>GEDPQTFEGAGVVFEVQVEKNLVDIDHRLYRLPNSTVRNGMPSLFQVKPGSVVSYSGTVSQPWSTITDIYIH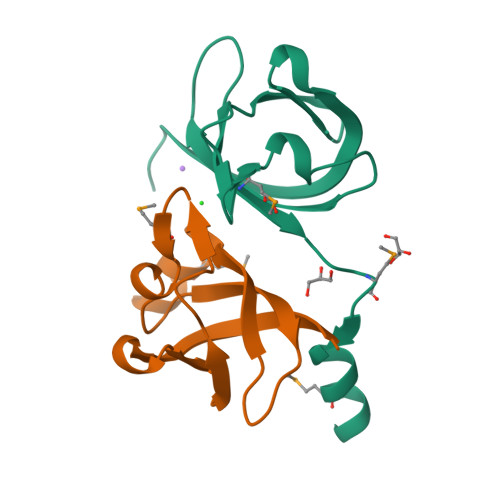KQMSEQELAEMIEKEQPRQDGEEQPR[2x]> MASAHIALELDKTKVKVGDVIVATVKAKNMTSMAGIQVNIKYDPEVLQAIDPATGKPFTKETLLVDPELLSNREYNPLLTAVNDINSGI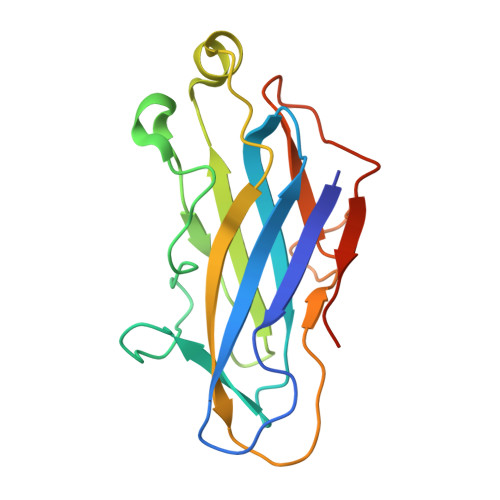INYASCYVYWDSYRESGVSESTGIIGKVGFKVLKAANTTVKLEETRFTPNSIDGTLVIDWYGQQIVGYKVIQPDLEHHHHHH>[2x]GPAMATNGEIFNTYGHNHQSATVTKITASNESSNGVCYLSETANLGKLICIPMALRAAMELNVFQLISKFGTDAKVSASEIASKMPNAKNNPEAAMYLDRILRLLGASSILSVSTTAASINRGGDDVVVHEKLYGLTNSSCCLVPRQEDGVSLVEELLFTSDKVVVDSFFKLKCVVEEKDSVPFEVAHGAKIFEYAA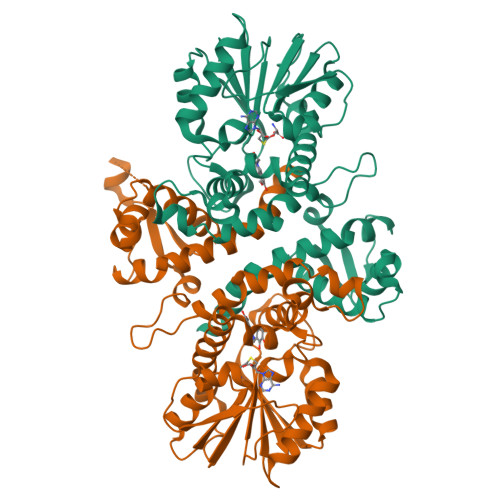TEPRMNQVFNDGMAVFSIVVFEAVFRVYDGFLDMKELLDVGGGIGTSVSKIVAKYPLIRGVNFDLPHVISVAPQYPGVEHVAGDMFEEVPKGQNMLLKWVLHDWGDERCVKLLKNCWNSLPVGGKVLIIEFVLPNELGNNAESFNALIPDLLLMALNPGGKERTISEYDDLGKAAGFIKTIPIPISNGLHVIEFHK>UGUGGUUCGCAACCAUCCCACAUAAAAAA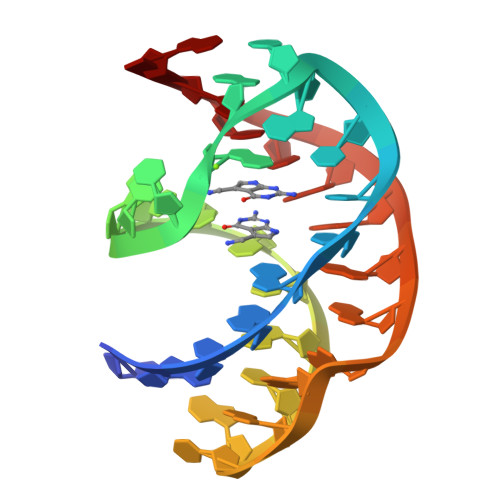ACUAG[3x]>MSAEEDARWLRWVTQQFKTIAGEDGEISLQEFKAALHVKESFFAERFFALFDSDRSGTITLQELQEALTLLIHGSPMDKLKFLFQVYDIDGSGSIDPDELRTVLQSCLRESAISLPDEKLDQLTLALFESADADGNGAITFEELRDELQRFPGVMENLTISAAHWLTAPAPRPRPRRPRQLTRAYWHNHRSQLFCLATYAGLHVLLFGLAASAHRDLGASVMVAKGCGQCLNFDCSFIAVLMLRRCLTWLRATWLAQVLPLDQNIQFHQLMGYVVVGLSLVHTVAHTVNFVLQAQAEASPFQFWELLLTTRPGIGWVHGSASPTGVALLLLLLLMFICSSSCIRRSGHFEVFYWTHLSYLLVWLLLIFHGPNFWKWLLVPGILFFLEKAIGLAVSRMAAVCIMEVNLLPSKVTHLLIKRPPFFHYRPGDYLYLNIPTIARYEWHPFTISSAPEQKDTIWLHIRSQGQWTNRLYESFKASDPLGRGSKRLSRSVTMRKSQRSSKGSEILLEKHKFCNIKCYIDGPYGTPTRRIFASEHAVLIGAGIGITPFASILQSIMYRHQKRKHTCPSCQHSWIEGVQDNMKLHKVDFIWINRDQRSFEWFVSLLTKLEMDQAEEAQYGRFLELHMYMTSALGKNDMKAIGLQMALDLLANKEKKDSITGLQTRTQPGRPDWSKVFQKVAAEKKGKVQVFFCGSPALAKVLKGHCEKFGFRFFQENF[2x]

NADPH oxidase 5 (NOX5) catalyzes the production of superoxide free radicals and regulates physiological processes from sperm motility to cardiac rhythm. NOX5 catalyzes the electron transfer from cytosolic NADPH to extracellular oxygen to produce superoxide (O2-) in the presence of intracellular Ca2+ ions. Like DUOX1-2, Ca2+ activates NOX5 by binding to its regulatory EF-hand domain (EFD). Each protomer contains a catalytic core with TMD, FBD and NBD and a regulatory EFD.

In the consensus structure of intermediate state (Ca2+- and NADPH-bound NOX5) determined at an overall resolution of 3.3 Å with C2 symmetry, the EFD was not resolved due to its flexibility. To analyze the EFD motion, we performed 3D classification and refinement without applying symmetry and identified at least three distinct conformations (intermediate state 1–3) with large spatial displacement. The local resolutions of EFD in intermediate state 1 and 2 are insufficient for modeling secondary structure, whereas the intermediate state 3 was resolved to an overall resolution of 3.9 Å, enabling the model building of EFD. These conformations, with the EFDs manifesting a trajectory towards the membrane, could represent its motions during NOX5 activation process. The EFD moves toward the membrane upon Ca2+ activation, shortening the distance by more than 12 Å between EFD and TMD. The preTM1 helix, which caps the NADPH-binding pocket, uplifts. The NBD shows a minor displacement coupled to the movement of the REFBD motif. These conformational changes synergistically remodel the NADPH-binding pocket by enlarging the binding site and altering the local surface potential. Finally, the nicotinamide moiety of NADPH shows a weak density in the intermediate state 3 structure, suggesting the flexibility of this moiety as observed in the mouse DUOX1 structure. In addition, the PhosR region becomes flexible and not visible upon Ca2+ binding.>[3x]GASPSAQELKEQGNRLFVGRKYPEA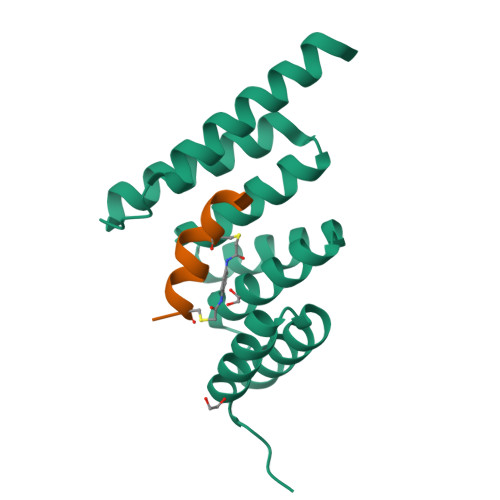AACYGRAITRNPLVAVYYTNRALCYLKMQQHEQALADCRRALELDGQSVKAHFFLGQCQLEMESYDEAIANLQRAYSLAKEQRLNFGDDIPSALRIAKKKRWNSIEERR;>[3x]XPWWECLSQADDCDFRX>[2x]MSDKDSKNTPQVPEK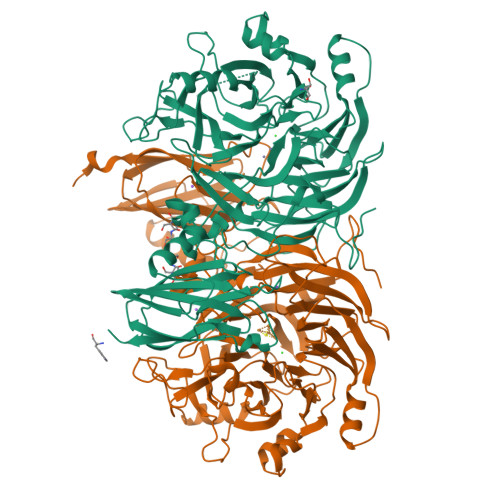LGLSRRGFLGASAVTGAAVAATALGGAVMTRESWAQAVKESKQKIHVGPGELDDYYGFWSGGHQGEVRVLGVPSMRELMRIPVFNVDSATGWGLTNESRHIMGDSAKFLNGDCHHPHISMTDGKYDGKYLFINDKANSRVARIRLDIMKCDKMITVPNVQAIHGLRLQKVPHTKYVFANAEFIIPHPNDGKVFDLQDENSYTMYNAIDAETMEMAFQVIVDGNLDNTDADYTGRFAAATCYNSEKAFDLGGMMRNERDWVVVFDIHAVEAAVKAGDFITLGDSKTPVLDGRKKDGKDSKFTRYVPVPKNPHGCNTSSDGKYFIAAGKLSPTCSMIAIDKLPDLFAGKLADPRDVIVGEPELGLGPLHTTFDGRGNAYTTLFIDSQVVKWNMEEAVRAYKGEKVNYIKQKLDVHYQPGHLHASLCETNEADGKWLVALSKFSKDRFLPVGPLHPENDQLIDISGDEMKLVHDGPTFAEPHDCIMARRDQIKTKKIWDRNDPFFAPTVEMAKKDGINLDTDNKVIRDGNKVRVYMTSMAPAFGVQEFTVKQGDEVTVTITNIDQIEDVSDGFVVVNHGVSMEISPQQTSSITFVADKPGLHWYYCSWFCHALHMEMVGRMMVEPAWSHPQFEK>[2x]QIQKAEQNDVKLAPPTDVRSGYIRLVKNVNYYIDSESIWVDNQEPQIVHFDAVVNLDKGLYVYPEPKRYARSVRQYKILNCANYHLTQVRTDFYDEFWGQGLRAAPKKQKKHTLSLTPDTTLYNAAQIICANYGEAFSVDKKGGTKKAAVSELLQASAPYKADVELCVYSTNETTNCTGGKNGIAADITTAKGYVKSVTTSNGAITVKGDGTLANMEYILQATGNAATGVTWTTTCKGTDASLFPANFCGSVTQGGHHHHHH

In the present study, a vaccine antigen based on the fusion of two known NTHi adhesive proteins, protein E (PE) and a pilin subunit (PilA), was developed. PE is a ubiquitous NTHi antigen described to be important for the adhesion of the bacterium to epithelial cells. It is also known to bind vitronectin, which protects the bacterium from complement attack, and immunization with a fragment of PE was shown to afford protection in a mouse model of pulmonary clearance. PilA is another ubiquitous NTHi antigen described to be a conserved protein among H. influenzae isolates. It is the major subunit of type IV pili (Tfp), which are hair-like filaments involved in adherence through ICAM-1 (25).

The construct produced in this study was a fusion protein composed of a large part of the PE sequence, a hinge of two glycines, and a large part of the PilA sequence. The crystal structure of the PE-PilA fusion protein showed that most of the protein was visible, except for three small disordered regions comprising the first seven N-terminal residues (in the PE domain), the linker region (residues 136 to 143), and the C-terminal His tag. PE-PilA also crystallized in space group C2 and had two molecules in the asymmetric unit with a noncrystallographic symmetry dimer interface (area, ∼450 Å2) via the PE domain of the fusion protein C terminus. Interestingly, crystal packing analysis revealed a crystallographic 2-fold PE domain dimer, very similar to the one observed in the isolated PE crystal form, with a comparable dimerization interface area (∼870 Å2). It is unclear whether this crystallographic dimer represents the biological dimer, but it probably represents a favored interface in the crystallization process. The PE and PilA entities of the PE-PilA crystal structure have tertiary structures that closely match the isolated PE crystal structure and PilA homology model, respectively. In addition, two disulfide bridges in the PilA domain of the fusion protein that corroborate the mass spectrometry data were revealed; one (Cys167-Cys177) links the N-terminal α-helix to the intervening loop of the first β-strand, and the other (Cys236-Cys249) links the final β-strand to the C-terminal loop. Only the N-terminal hydrophobic α-helix tail was missing in our tethered PilA, but this tail provides both an anchor for the globular head and a hydrophobic surface for the assembly of pilin subunits to form a pilus and as such seems less accessible to antibodies than the globular head and, thus, less immunologically relevant. We observed a more substantial crystallographic symmetry dimer interface (∼870 Å2) in PE-PilA via the PE domain and one of ∼890 Å2 for the isolated PE (excluding the C-terminal His tag). Interestingly, our PE dimers were generated at pH 4 to 4.5, close to the side chain pKa of the key interacting residues Asp52 and Glu54, while the published structure was obtained at pH 6.0.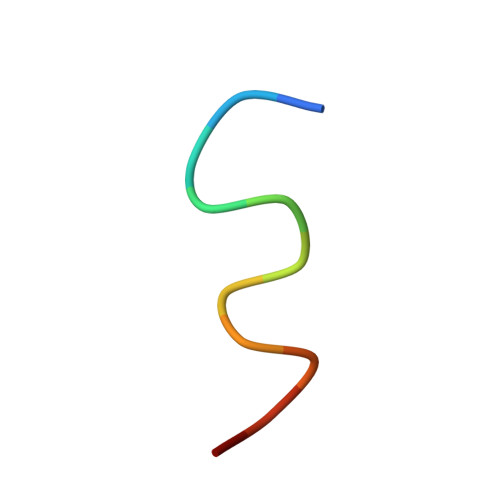> KKLLKLLKLLLX In this study, we report the synthesis of 2′-formamidonucleoside phosphoramidite derivatives and their incorporation into siRNA strands to reduce seed-based off-target effects of small interfering RNAs (siRNAs). While 2′-formamidonucleotide triphosphate and nucleosides have been synthesized previously, their incorporation into oligonucleotides has not been reported, leaving their physical properties unknown. Introducing these derivatives into double-stranded RNA slightly reduced its thermodynamic stability, but X-ray crystallography and CD spectrum analysis confirmed that the RNA maintained its natural A-form structure. Although the introduction of the 2′-formamidonucleoside derivative at the 2nd position in the guide strand of the siRNA led to a slight decrease in the on-target RNAi activity, the siRNAs with different sequences incorporating 2′-formamidonucleoside with four kinds of nucleobases into any position other than 2nd position in the seed region revealed a significant suppression of off-target activity while maintaining on-target RNAi activity. This indicates that 2′-formamidonucleosides represent a promising approach for mitigating off-target effects in siRNA therapeutics.

Notably, the introduction of 5-bromouridine allows the bromine atom to act as an anomalous scatterer, enabling structural determination via anomalous dispersion methods.

>GGACUCGAGXCC[2x]> SVSDTNLYSPFKPRNYQLELALPAMKGKNTIICAPTGCGKTFVSLLICEHHLKKFPQGQKGKVVFFANQIPVYEQQKSVFSKYFERHGYRVTGISGATAENVPVEQIVENNDIIILTPQILVNNLKKGTIPSLSIFTLMIFDECHNTSKQHPYNMIMFNYLDQKLGGSSGPLPQVIGLTASVGVGDAKNTDEALDYICKLCASLDASVIATVKHNLEELEQVVYKPQKFFRKVESRISDKFKYIIAQLMRDTESLAKRICKDLENLSQIQNREFGTQKYEQWIVTVQKACMVFQMPDKDEESRICKALFLYTSHLRKYNDALIISEHARMKDALDYLKDFFSNVRAAGFDEIEQDLTQRFEEKLQELESVSRDPSNENPKLEDLCFILQEEYHLNPETITILFVKTRALVDALKNWIEGNPKLSFLKPGILTGRGKTNQNTGMTLPAQKCILDAFKA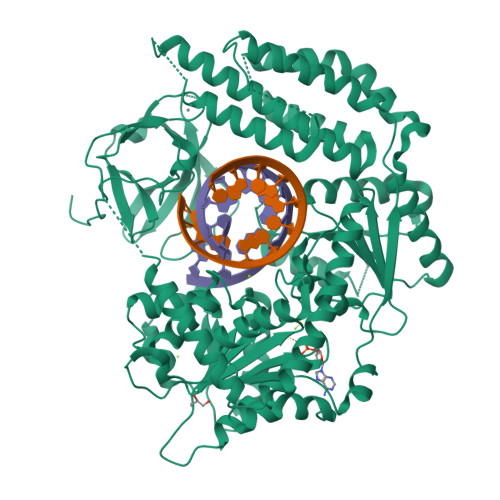SGDHNILIATSVADEGIDIAQCNLVILYEYVGNVIKMIQTRGRGRARGSKCFLLTSNAGVIEKEQINMYKEKMMNDSILRLQTWDEAVFREKILHIQTHEKFIRDSQEKPKPVPDKENKKLLCRKCKALACYTADVRVIEECHYTVLGDAFKECFVSRPHPKPKQFSSFEKRAKIFCARQNCSHDWGIHVKYKTFEIPVIKIESFVVEDIATGVQTLYSKWKDFHFEKIPFDPAEMSK>[4x]STVYNINLGIGWASSGVEYAQAYRAQILRRIQQPAKFIFMDMILADNIQHLTENIGFLDEEIIWLYNYFTDIKIAPTTVTLDQVLAQVAGQPERSEKEGKIVRYFYPQDDQFITCYLRQEDQDFVEHVEYVSRGRLIRKDYFSYVRYASEYFAPHNDAATLYQRRFYHEDGSVAYDMLIEDGQEKLYRFPDRIFYSKAELVRYFLQCLQLQADDVVILDRETGIGQ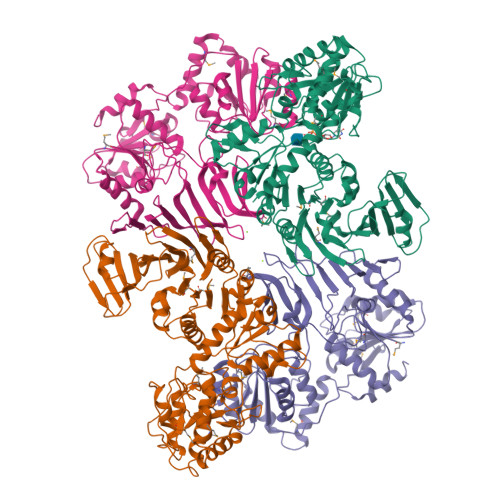VVFEESQKAKLGVVVHAEHFSENASSDDYILWNNFYDYQFTNADKVDFFIVATEAQKRILEQQFQHYSDKQPQIATIPVGSLDQLTYPKEPRKPYSMITASRLATEKHIDWLVAATVQAHAQLPELTLDIYGKGSEEDKLRRRIEEAGAQDYIRLKGHADLSQIYAGYELYLTASTSEGFGLTLMEAVGSGLPLIGFDVRYGNQTFIDDGKNGYLLPVSSNHVEDQIIAAFVEKIIALFSQGRQQEMSQHSYQVAENYLTSRVEAAWTQLLKEVRDD;>[4x]MIQLFDYYNQETQDLHDSLLAAGYACPTIVIEANGFLPDDMISPYTYFLGDEEGVDHPLFFNQVPVPPFWEITGDHQVARVSDMGEERARIHYASQARGRLVKQVDWLDKKGQLRLSERYNKQGRCFAKTAYKSGQEAFNTTYYSTDGQERIVENHVTGDIILTLDQEPLRIFKSRVDFIRFFLERLDLDLDHILFNSLAYSFLVSHSLTGRAGQDILFWQEPLYDELPGNMQLILDNSQLRTQTIVIPDLATYEKAMSLAAADQQQKFLHLGYHYDFKRDNYLRKDALILTHSDQIEGLDTLVQSLPQLVFRIAALTEMSPKLLSMLSYKNVVLYQNASLKQIEQLYLESDIYLDINHGGQVLQAVRKAFENNLLILGFEQTLHDRHYIAQQHIFDSSQPAQLASILEEALCGVEQMRSALQAQGRHANDVPVSLYQETLQSLLG demethylated cyclopeptin | C16 H14 N2 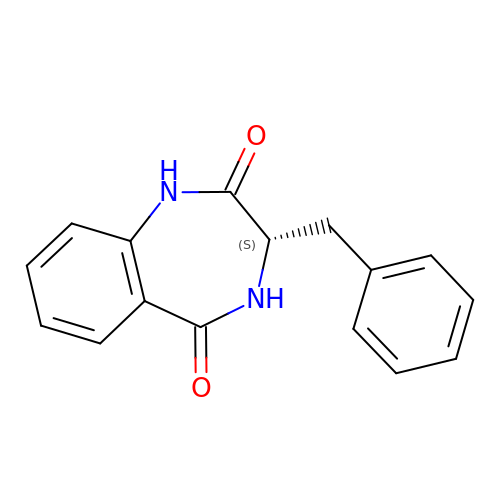O2 | IOYQGXYNQRRATP-AWEZNQCLSA-N>VIEKVQHIQLLQKNVRAQLVDMKRLEVDIDIKIRSCRGSCSRALAREVDLKDYEDQQKQLEQVIAK[2x];>[2x]HQLYIDETVNSNIPTNLRVLRSILENLRSKIQKLESDVSAQMEYCRTPCTVSCNIPVVSGKECEEIIRKGGETSEMYLIQPDSSVKPYRVYCDMNTENGGWTVIQNRQDGSVDFGRKWDPYKQGFGNVATNTDGKNYCGLPGEYWLGNDKISQLTRMGPTELLIEMEDWKGDKVKAHYGGFTVQNEANKYQISVNKYRGTAGNALMDGASQLMGENRTMTIHNGMFFSTYDRDNDGWLTSDPRKQCSKEDGGGWWYNRCHAANPNGRYYWGGQYTWDMAKHGTDDGVVWMNWKGSWYSMRKMSMKIRPFFPQQ;>YEASILTHDSSIRYLQEIYNSNNQKIVNLKEKVAQLEAQCQEPCKDTVQIHDITGKDCQDIANKGAKQSGLYFIKPLKANQQFLVYCEIDGSGNGWTVFQKRLDGSVDFKKNWIQYKEGFGHLSPTGTT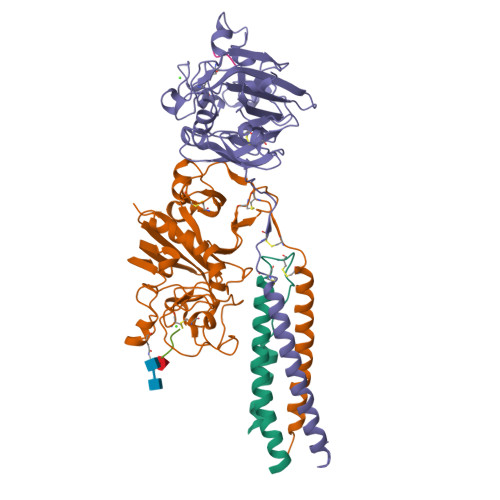EFWLGNEKIHLISTQSAIPYALRVELEDWNGRTSTADYAMFKVGPEADKYRLTYAYFAGGDAGDAFDGFDFGDAPSAKFFTSHNGMQFSTWDNDNDKFEGNCAEQDGSGWWMNKCHAGHLNGVYYQGGTYSKASTPNGYDNGIIWATWKTRWYSMKKTTMKIIPFNRLTIGEGQQHHLGGAK[2x];>GHRP[4x]> KKAVPYNRMKLMIVGNTGSGKTTLLQQLMKTKKSDLGMQSATVGIDVKDWPIQIRDKRKRDLVLNVWDFAGREEFYSTHPHFMTQRALYLAVYDLSKGQAEVDAMKPWLFNIKARASSSPVILVGTHLDVSDEKQRKACMSKITKELLNKRGFPAIRDYHFVNATEESDALAKLRKTIINESLNFKIRDQLVVGQLIPDCYVELEKIILSERKNVPIEFPVIDRKRLLQLVRENQLQLDENELPHAVHFLNESGVLLHFQDPALQLSDLYFVEPKWLCKIMAQILTVKVEGCPKHPKGIISRRDVEKFLSKKRKFPKNYMSQYFKLLEKFQIALPIGEEYLLVPSSLSDHRPVIELPHCENSEIIIRLYEMPYFPMGFWSRLINRLLEISPYMLSGRERALRPNRMYWRQGIYLNWSPEAYCLVGSEVLDNHPESFLKITVPSCRKGCILLGQVVDHIDSLMEEWFPGLLEIDICGEGETLLKKWALYSFNDGEEHQKILLDDLMKKAEEGDLLVNPDQPRLTIPISQIAPDLILADLPRNIMLNNDELEFEQAPEFLLGDGSFGSVYRAAYEGEEVAVKIFNKHTSLRLLRQELVVLCHLHHPSLISLLAAGIRPRMLVMELASKGSLDRLLQQDKASLTRTLQHRIALHVADGLRYLHSAMIIYRDLKPHNVLLFTLYPNAAIIAKIADYGIAQYCCRMGIKTSEGTPGFRAPEVARGNVIYNQQADVYSFGLLLYDILTTGGRIVEGLKFPNE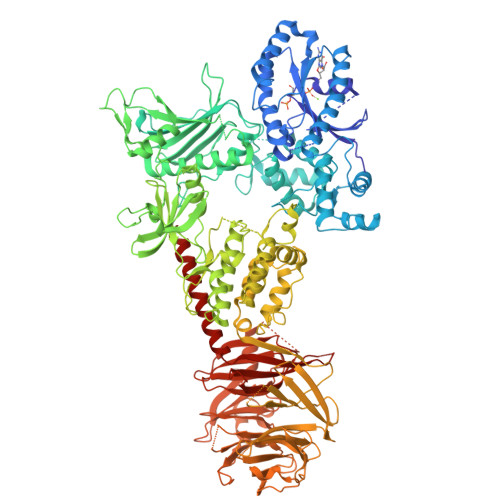FDELEIQGKLPDPVKEYGCAPWPMVEKLIKQCLKENPQERPTSAQVFDILNSAELVCLTRRILLPKNVIVECMVATHHNSRNASIWLGCGHTDRGQLSFLDLNTEGYTSEEVADSRILCLALVHLPVEKESWIVSGTQSGTLLVINTEDGKKRHTLEKMTDSVTCLYCNSFSKQSKQKNFLLVGTADGKLAIFEDKTVKLKGAAPLKILNIGNVSTPLMCLSESTNSTERNVMWGGCGTKIFSFSNDFTIQKLIETRTSQLFSYAAFSDSNIITVVVDTALYIAKQNSPVVEVWDKKTEKLCGLIDCVHFLREVMVKENKESKHKMSYSGRVKTLCLQKNTALWIGTGGGHILLLDLSTRRLIRVIYNFCNSVRVMMTAQLGSLKNVMLVLGYNRKNTEGTQKQKEIQSCLTVWDINLPHEVQNLEKHIEVRKELAEKMRRTSVE>[2x]AEPFAKLEQDFGGSIGVYAMDTGSGATVSYRAEERFPLCSSFKGFLAAAVLARSQQQAGLLDTPIRYGKNALVPWSPISEKYLTTGMTVAELSAAAVQYSDNAAANLLLKELGGPAGLTAFMRSIGDTTFRLDRWELELNSAIPSDARD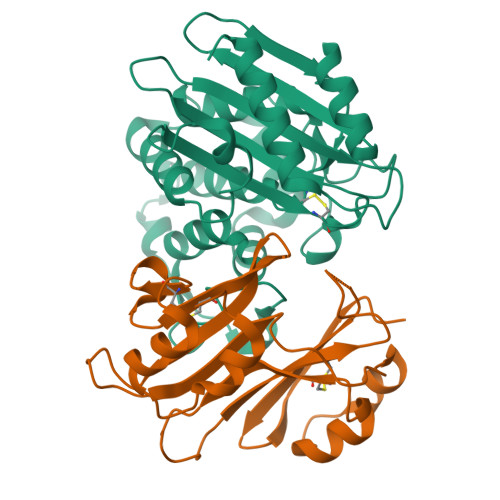TSSPRAVTESLQKLTLGSALAAPQRQQFVDWLKGNTTGNHRIRAAVPADWAVGDKTGTCGVYGTANDYAVVWPTGRAPIVLAVYTRAPNKDDKHSEAVIAAAARLALEGLGVNGQ;>AGVMTGAKFTQIQFGMTRQQVLDIAGAENCETGGSFGDSIHCRGHAAGDYYAYATFGFTSAAADAKVDSKSQEKLLAPSAPTLTLAKFNQVTVGMTRAQVLATVGQGSCTTWSEYYPAYPSTAGVTLSLSCFDVDGYSSTGFYRGSAHLWFTDGVLQGKRQWDLV[2x]>[4x]MGHHHHHHSAPMMSTHLADRYNQAWLFAARAHRNQTLSGSPLP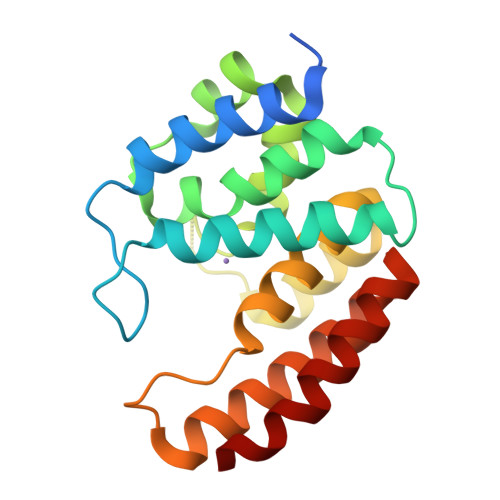YLVHLGMVANELLAADRDGAIERLGETLQIAVLHDTLEDTATSPEELRQQFGEFVCAGVQALSKRVGDGPKRSLDDYLQALAEGPAQYALVKLCDRITNLQPPPQTWNQDKIANYHQESQLILARLGHAHAATARRLREKIEHYRQYY>[4x]MEIVAPVITTFRGGRLDPELFANHVKNITSKGVDVVFVAGTTGLGPALSLQEKMELTDAATSAARRVIVQVASLNADEAI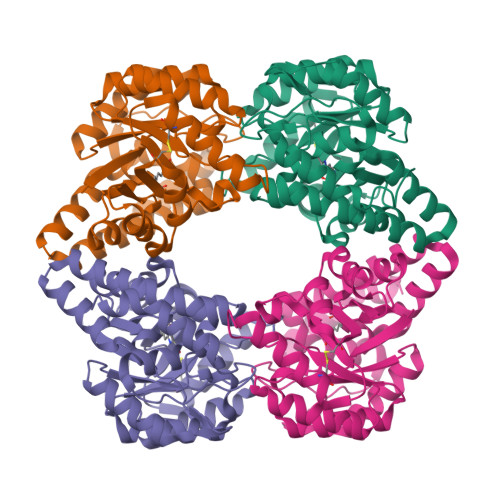ALAKYAESRGAEAVASLPPYYFPRLSERQIAKYFRDLCSAVSIPVFLYNYPAAVGRDVDARAAKELGCIRGVKDTNESLAHTLAYKRYLPQARVYNGSDSLVFASFAVRLDGVVASSANYLPELLAGIRDAVAAGDIERARSLQFLLDEIVESARHIGYAAAVYELVEIFQGYEAGEPRGPVYPLDPEEKAWLRAAVAKAKSQLRL> MAESKPTPQSTFTGPIVVDPITRIEGHLRIMVEVENGKVKDAWSSSQLFRGLEIILKGRDPRDAQHFTQRACGVCTYVHALASSRCVDDAVKVSIPANARMMRNLVMASQYLHDHLVHFYHLHALDWVDVTAALKADPNKAAKLAASIAPARPGNSAKALKAVQDKLKAFVESGQLGIFTNAYFLGGHKAYYLPPEVDLIATAHYLEALHMQVKAASAMAILGGKNPHTQFTVVGGCSNYQGLTKDPLANYLALSKEVCQFVNECYIPDLLAVAGFYKDWGGIGGTSNYLAFGEFATDDSSPEKHLATSQFPSGVITGRDLGKVDNVDLGAIYEDVKYSWYAPGGDGKHPYDGVTDPKYTKLDDKDHYSWMKAPRYKGKAMEVGPLARTFIAYAKGQPDFKKVVDMVLGKLSVPATALHSTLGRTAARGIETAIVCANMEKWIKEMADSGAKDNTLCAKWEMPEESKGVGLADAP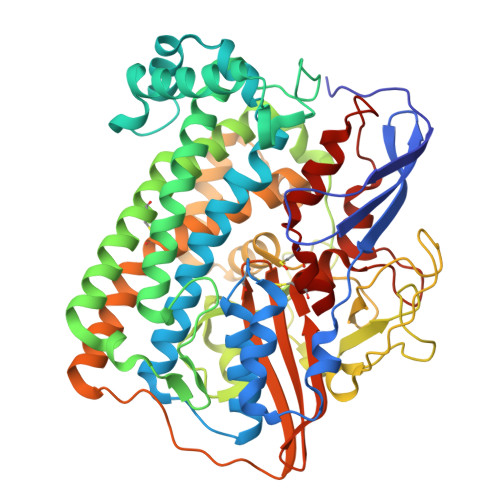RGALSHWIRIKGKKIDNFQLVVPSTWNLGPRGAQGDKSPVEEALIGTPIADPKRPVEILRTVHAFDPCIACGVH> MQPVVLRGISSLTWQHARGALPSALQQALAASAASSSSSLTAVDCDAGADMQASCSGRGVECARHRLAWGPLSGVAGLSTSARAASPAAAAMPSSSAASAASPAADAAPPGAYSVEIAVQGFEKRYVDMACNTLGDIIILAFAPKSYAALPTGAPSPSDAPVNLAFGPERRDVRLPWRRTRITLIRGPHIDKTGMEQFERREYKSVLTAATNCPQELARLLEAVKLYQFTGVQIKMQLASAQRVDLPADVSALLRGGGGATAASTGSSSSSSSSSSSSSSLVGSPVVXXXXXXXXXXXXXXXXXXXXXXXXXXXXXXXXEIPAPASADLAFAEEVGRVLGVLRPAVWAGLSRRRAVLAGSADHETWLKAAAGGLPPSASATRGAGRGGGAA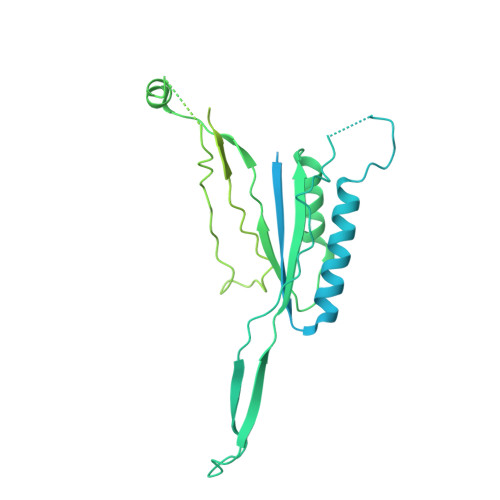ALPPPAVVAGWDAEAEVAGAAAEGGDAFGRLLRLRLRQQAQLQDAQASTSASGTSTPAAASAAAYGLDPALAARLLARIDADLLHAHEAAAAGLPPPAALAAGTAAAAVAAPPPATAVLDASKMSPAEYAYAVLKYVQYVDSLYESSGAAAAAARGDAALQLAAPALAVRLLQLWWEATTVEFKRALGLPPAEEERRMLERLLELQKKKDELKGAGRGGGR Here, we have solved by X-ray crystallography the structure of methylenetetrahydrofolate dehydrogenase (MTHFD) from Thermus thermophilus. This organism is an extreme thermophilic model organism, which has been described as having an optimal growth ranging from 65°C to 72°C and being resistant to maximum temperatures of 85°C. MTHFD is a key enzyme in the folate-dependent one carbon metabolism, which is important for the biosynthesis of several amino acids like glycine, alanine and serine, as well as nucleotide bases, formylated methionine and some pro-vitamins. In some bacteria like E. coli, MTHFD (called FolD in this species) is a dual function enzyme that catalyzes the conversion of 5,10‐methylenetetrahydrofolate and NADP+ to 5,10-methenyltetrahydrofolate and NADPH (dehydrogenase function), and further converts the first product to 10-formyltetrahdrofolate (cyclohydrolase function).

The final model included one chain of TtMTHFD, one NADP+ nucleotide molecule and 60 water molecules in the asymmetric unit. TtMTHFD consists of two α/β-fold sub-domains connected by two large α-helices, which are at the same time the N-terminal and C-terminal α-helices. The N-terminal α/β-fold sub-domain is the catalytic domain that binds the main substrate, and the C-terminal α/β-fold sub-domain is the nucleotide (co-substrate) binding domain, which are variants of the structurally conserved Rossmann dinucleotide-binding domain fold. Both domains are interconnected by an extended loop-helix-loop motif that we here termed ‘Connector Helix (CH) region’. Compared to the Thermoplasma acidophilum MTHFD (TaMTHFD) and Acinetobacter baumannii MTHFD (AbMTHFD) structures, T. thermophilus MTHFD (TtMTHFD) showed an overall RMSD of 0.98 Å (with an overall sequence identity of 36%) and an overall RMSD of 1.29 Å (with an overall sequence identity of 39%), respectively. Conversely, using a cut-off value of 4 Å, a higher amount of salt-bridges in the crystal structure of TtMTHFD (n = 26), when compared with TaMTHFD (n = 16) and AbMTHFD (n = 10), could be identified. Interestingly, again TtMTHFD showed a higher number of inter-chain salt bridges (n = 6) in comparison with TaMTHFD (n = 2) and AbMTHFD (none), indicating the importance of salt bridges for the thermo-stabilization of dimers. Furthermore, TtMTHFD had a higher number of arginine-formed salt-bridges (n = 23) compared with TaMTHFD (n = 5) and AbMTHFD (n = 6), as expected for thermophilic proteins. Thus, an important conclusion is that in TtMTHFD a large amount of salt bridges probably contributes both statically, i.e. through more elevated Coulomb interactions, as well as dynamically, through higher energy dissipation capabilities, to the stabilization of the protein.

> MAAQVLSGHEAAEAVYEEIRARLRSLSFTPSLRVIRLGEDPASVAYVRLKDKRARALGYRSQVEVYPEDLPEEALLERIAALNADEEVDGILVQLPLPPHIRTQRVLEAIHPLKDVDGFHPLNVGRLWSGGKGLFPCTPLGVVRLLKHYGVDLRGKEVVVVGRSNIVGKPLAGLLLREDATVTLAHSKTQDLPEVTRRAQVLVVAVGRPHLVRKEWVREGAIVVDVGVNRVEGRLLGDVHPEVAEVAFALTPVPGGVGPMTVAMLMGNTLEAALLRR>MGHHHHHHSAISVWRAVDYVRMPWKNGGGSTEEITRDAGTGLEGFGWRLSIADIGESGGFSSFAGYQRVITVIQGAGMVLTVDGEEQRGLLPLQPFAFRGDSQVSCRLITGPIRDFNLIYSPERYHARLQWVDGVQ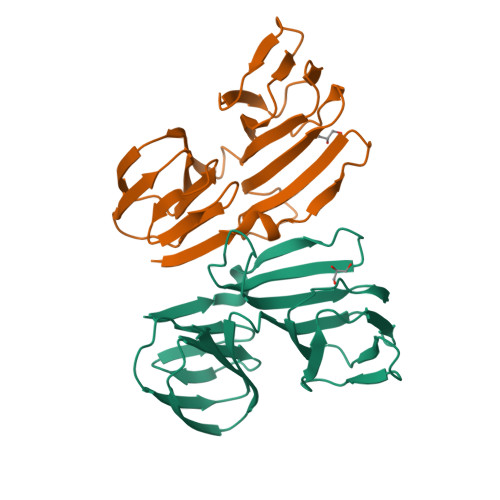RFFSTAQTVLVFSVADEVKVLGEKLGHHDCLQVDGNAGLLDISVTGRCCLIELTQRG[2x]>GSHMTHASDSGSSRWSKDYDVCVCHSEEDLVAAQDLVSYLEGSTASLRCFLQLRDATPGGAIVSELCQALSSSHCRVLLITPGFLQDPWCKYQMLQALTEAPGAEG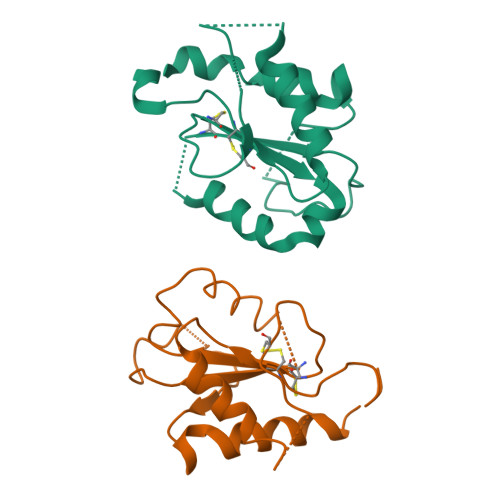CTIPLLSGLSRAAYPPELRFMYYVDGRGPDGGFRQVKEAVMRYLQTLS[2x]> MVAPEHRVLHLRDRLDLAAELKLLCERGPLVRIPLEDGSAVHWFALGYDVVREVLGSEKFDKRVIGTHFNHQEMALPGNLLQLDPPEHTRLRRMVAPAFSVRRMQALEPRVQAIVDDHLDTMASTGPPVEFLREVAGPMAARVACEFLGIPLDDRGELIRLTAHRGGKRRRVLNGHAYLAYMRELAARLRRDPGDGMLGMVARDHGADISDEELAGLCAVVMNSSVEQTESCLAAGTLLLLEHPEQFALLRERPELGEQAVEEIVRYLSVFEGLDPRTATEDVEIGGQVIKKGEAVFCSLLAANRADPALDGFDITRKESRHVAFGHGIHHCLGAPLARMELRIAFTTLVSRFPSLRTAVPAEEIRFRPPSSNVFTLLELPLTW

Cytochrome P450 enzymes (P450s) are a superfamily of monooxygenases that utilize a cysteine thiolate–ligated heme moiety to perform a wide range of demanding oxidative transformations. Within GPA biosynthesis, P450s function in a specific, stepwise manner to install the essential side-chain crosslinks in the core peptide in a process that typically requires one Oxy enzyme per crosslink to be installed. Given the apparent preference for the unusual heme orientation shown by OxyA enzymes, we investigated the OxyA homolog from kistamicin biosynthesis (OxyAkis), which is an atypical GPA. Structural and biochemical analysis of OxyAkis has shown that this P450 enzyme is highly prone to oxidation and can display an atypical heme orientation in different protein batches.

The tyrosine residue at position 99 (position 119 in the His-tagged OxyAkis protein) is oriented in such a way that the phenol moiety is very close to the site of additional density present in the OxyAkis structure (distance from the phenol to the site of damage is 3.7 Å). As the phenol group present in Tyr99 appeared to be appropriately positioned to play a role in potential oxidative heme damage in the catalytic site of OxyAkis, we next cloned a mutant in which Tyr99 was mutated into Phe by site-directed mutagenesis. The addition of H2O2 revealed that the mutant enzyme was slightly more stable to oxidative damage than the wild-type enzyme, although the mutant still exhibits the shoulder between 600 and 700 nm and is more sensitive to oxidizing agents than OxyCkis. To examine this mutant further, OxyAkis-Y99F was crystallized under the same conditions used for the native OxyAkis. These crystals, which are diffracted to a resolution of 1.8 Å, showed a mixed population of heme orientations in the enzyme active site (6:1 normal orientation/flipped orientation). Interestingly, no additional density has been observed at the β-position of the heme moiety as had been previously observed with the WT crystals. We observed weak and somewhat distorted electron density for the mutated phenylalanine residue itself, suggesting that the side chain exists in multiple conformations in the structure. Furthermore, it appears that residues 223–228 of the I-helix now adopt two conformations above the heme moiety. In the wild-type structure, a network of hydrogen bonding is observed between the Tyr99 phenol moiety and amide backbone of the I-helix residue Leu217, mediated via two water molecules. The Tyr99Phe mutation results in the loss of this H-bond network, which we then attribute to the differences seen in the structure by permitting both the increase in flexibility of the Phe99 side chain and further the second conformation adopted by the I-helix.> MTLSILVAHDLQRVIGFENQLPWHLPNDLKHVKKLSTGHTLVMGRKTFESIGKPLPNRRNVVLTSDTSFNVEGVDVIHSIE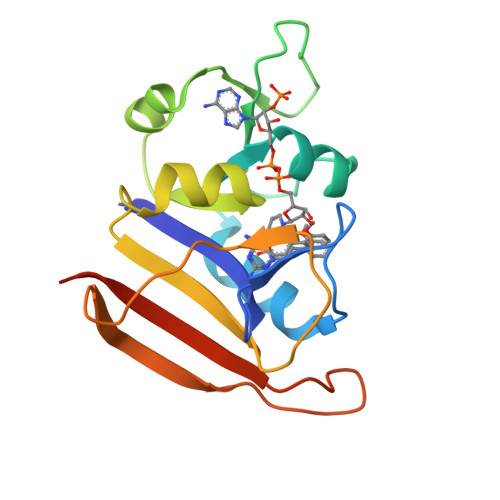DIYQLPGHVFIFGGQTLFEEMIDKVDDMYITVIEGKFRGDTFFPPYTFEDWEVASSVEGKLDEKNTIPHTFLHLIRKKLEHHHHHH>[4x]MPFAGSELP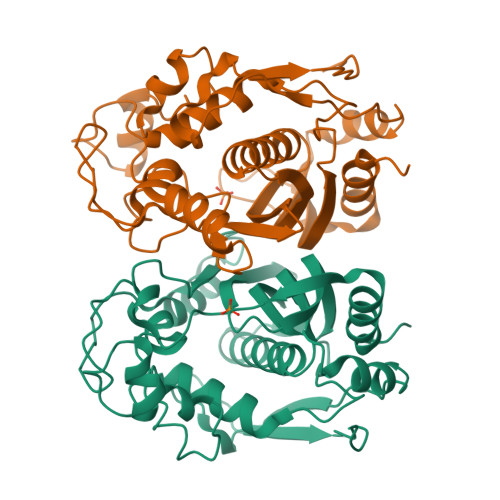RRPLPPAAQERDAEPRPPHGELQYLGQIQHILRCGVRKDDRTGTGTLSVFGMQARYSLRDEFPLLTTKRVFWKGVLEELLWFIKGSTNAKELSSKGVKIWDANGSRDFLDSLGFSTREEGDLGPVYGFQWRHFGAEYRDMESDYSGQGVDQLQRVIDTIKTNPDDRRIIMCAWNPRDLPLMALPPCHALCQFYVVNSELSCQLYQRSGDMGLGVPFNIASYALLTYMIAHITGLKPGDFIHTLGDAHIYLNHIEPLKIQLQREPRPFPKLRILRKVEKIDDFKAEDFQIEGYNPHPTIKMEMAV>APKAPADGLKMDKTKQPVVFNHSTHKAVKCGDCHHPVNGKEDYQKCATAGCHDNMD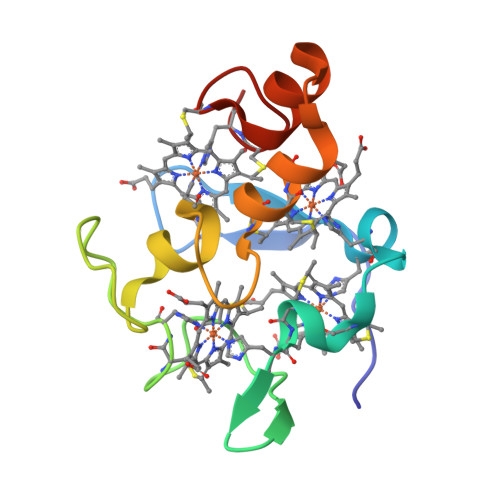KKDKSAKGYLHAMHDKGTKFKSCVGCHLETAGADAAKKKELTGCKGSKCHS[2x]> MQASQFSAQVLDWYDKYGR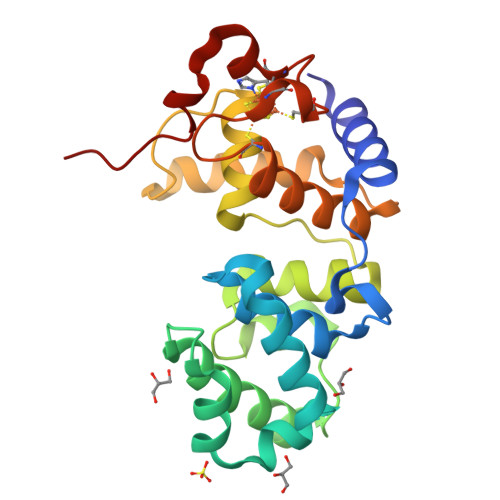KTLPWQIDKTPYKVWLSEVMLQQTQVATVIPYFERFMARFPTVTDLANAPLDEVLHLWTGLGYYARARNLHKAAQQVATLHGGKFPETFEEVAALPGVGRSTAGAILSLSLGKHFPILDGNVKRVLARCYAVSGWPGKKEVENKLWSLSEQVTPAVGVERFNQAMMDLGAMICTRSKPKHSLCPLQNGCIAAANNSWALYPGKKPK> MILGEIMEVLAFKNQSLIDHVNDMVKYWERIKYRYLKTIKRALEALNIKLDIEKVDEFMKILIKLHDIGKASKIYQRAIINDQEKLMGFRHELVSAYYTYHILLKKFGDKNLAFIGALTVMLHHEPIIMGQIRNLKKKELTAEVVLDKLKKFDGMIEDFEDLI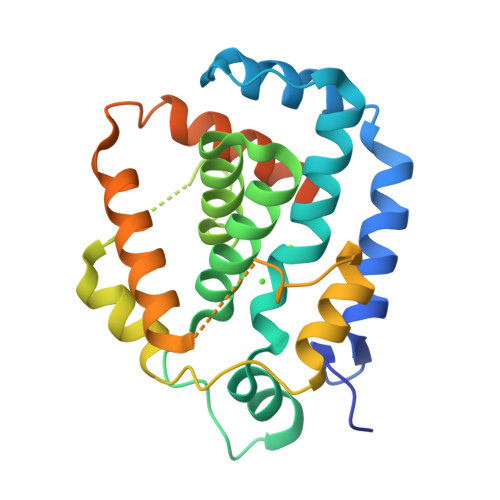KKLIGYSIGDIIKNDSNKDDIIRFVIEMSVRARHTPNSEKLRFIVGTLLLPLVMCDYKGAESREGKAPKFAEVLEVESYVI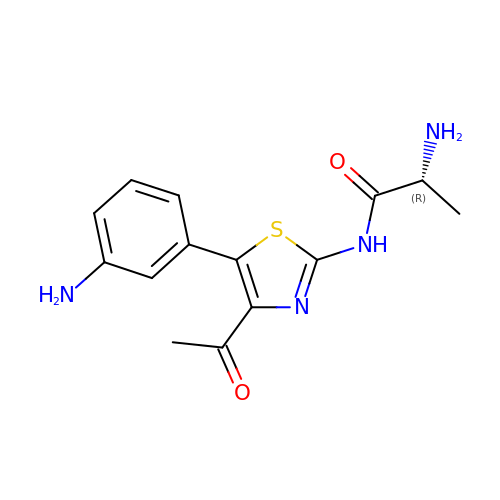(2~{R})-~{N}-[5-(3-aminophenyl)-4-ethanoyl-1,3-thiazol-2-yl]-2-azanyl-propanamide | C14 H16 N4 O2 S | NZFSZJLKZIHQBY-SSDOTTSWSA-N>GVFTFEDEITSTVPPAKLYNAMKDADSITPKIID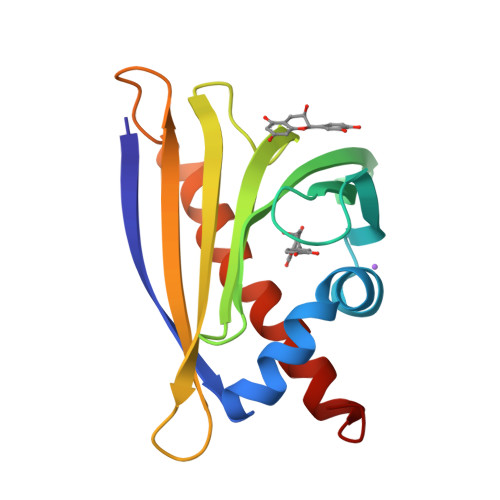DVKSVEIVEGNGGPGTIKKLTIVEDGETKFILHKVESIDEANYAYNYSVVGGVALPPTAEKITFETKLVEGPNGGSIGKLTLKYHTKGDAKPDEEELKKGKAKGEGLFRAIEGYVLANPTQY[4x]The enzyme serine hydroxymethyltransferase (SHMT) plays a key role in folate-mediated one carbon metabolism, providing precursors for multiple metabolic pathways. SHMT catalyzes the reversible conversion of L-serine and THF into glycine and 5,10-methylene THF. SHMT is highly conserved in evolution, utilizes pyridoxal 5-phosphate (PLP) as a co-factor and can accept polyGlu-THF as a substrate (Matthews et al., 1982; Schirch and Strong, 1989; Strong et al., 1989). Previous structural studies of soybean SHMT8 have provided detailed snapshots of the enzyme, representative of different stages of its multi-step reaction: the resting state of the enzyme with PLP; the enzyme bound to the PLP-Gly intermediate; and a ternary complex of the enzyme with PLP-Gly and the substrate analog FTHF (Korasick et al., 2020). These structures showed that, similar to SHMT from other eukaryotes, soybean SHMT8 adopts a tetrameric assembly, verified in solution by small-angle X-ray scattering and analytical ultracentrifugation (Korasick et al., 2020).

In this study, we have determined the crystal structure of soybean SHMT8 in complex with diGlu-FTHF and PLP-Gly at 1.7 Å resolution. A superposition of the polypeptide chains in FTHF and diGlu-FTHF complexes yields a Cα root mean square deviation (rmsd) of 0.48 Å over 1892 residues, highlighting their overall structural similarity. In the SHMT8 complex with diGlu-FTHF, we identify an additional conformational change of the THF-binding loop specifically associated with the presence of second glutamate moiety (Glu2) of the ligand. The loop closes in more tightly against the bound diGlu-FTHF. This is apparent from changes in the position of the backbone of 1-2 Å as well as in the sidechain of Leu383, a residue in the middle of the loop, which undergoes a significant rotation with a resulting change of ~5 Å in the position of the terminal carbon atoms. In the diGlu-FTHF complex, the Leu383 sidechain (chain A) packs against the ring of Tyr68 (chain B), making a potential CH – π hydrogen bond (Brandl et al., 2001). Another hydrogen bond is found between the sidechain of Ser381 and a backbone oxygen of Glu2. In addition, two hydrogen bonds are formed between the backbone amides of residues 382 and 383 and the γ-carbonyl of the first glutamate moiety (Glu1). A water-mediated contact is found between a carboxyl oxygen of Glu1 and the sidechain hydroxyl group of Tyr68.

>[4x]MGSSHHHHHHHSSGLVPRGSHMDPVSVWGNTPLATVDPEIHDLIEKEKRRQCRGIELIASENFTSFAVIEALGSALTNKYSEGMPGNRYYGGNEYIDQIENLCRSRALQAFHLDAQSWGVNVQPYSGSPANFAAYTAVLNPHDRIMGLDLPSGGHLTHGYYTSGGKKISATSIYFESLPYKVNSTTGYIDYDRLEEKALDFRPKLIICGGSAYPRDWDYKRFREVADKCGALLLCDMAHTSGLVAAQEVNSPFEYCDIVTTTTHKSLRGPRAGMIFYRKGPKPPKKGQPENAVYDFEDKINFAVFPSLQGGPHNHQIGALAVALKQAASPGFKAYAKQVKANAVALGKYLMGKGYSLVTGGTENHLVLWDLRPLGLTGNKVEKLCDLCNITVNKNAVFGDSSALAPGGVRIGAPAMTSRGLVEKDFEQIGEFLHRAVTLTLEIQKEHGKLLKDFNKGLVNNKAIEDLKADVEKFSALFDMPGFLVSEMKYKD> MSRQSISLRFPLLLLLLSPSPVFSADPGAPAPVNPCCYYPCQHQGICVRFGLDRYQCDCTRTGYSGPNCTIPEIWTWLRTTLRPSPSFIHFLLTHGRWLWDFVNATFIRDTLMRLVLTVRSNLIPSPPTYNIAHDYISWESFSNVSYYTRILPSVPRDCPTPMGTKGKKQLPDAEFLSRRFLLRRKFIPDPQGTNLMFAFFAQHFTHQFFKTSGKMGPGFTKALGHGVDLGHIYGDNLERQYQLRLFKDGKLKYQMLNGEVYPPSVEEAPVLMHYPRGIPPQSQMAVGQEVFGLLPGLMLYATIWLREHNRVCDLLKAEHPTWGDEQLFQTARLILIGETIKIVIEEYAQQLSGYFLQLKFDPELLFGAQFQYRNRIAMEFNQLYHFHPLMPDSFRVGPQDYSYEQFLFNTSMLVDYGVEALVDAFSRQPAGRIGGGRNIDHHILHVAVDVIKESRVLRLQPFNEYRKRFGMKPYTSFQELTGEKEMAAELEELYGDIDALE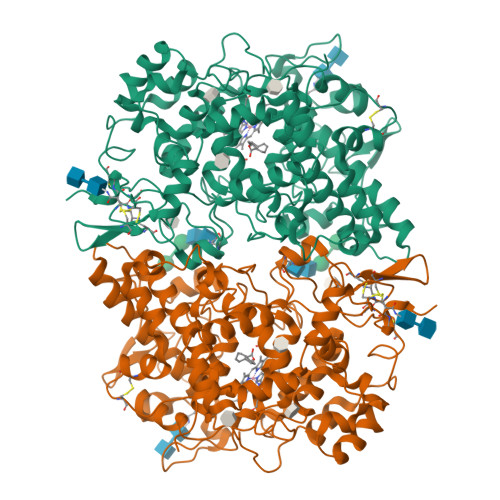FYPGLLLEKCHPNSIFGESMIEMGAPFSLKGLLGNPICSPEYWKASTFGGEVGFNLVKTATLKKLVCLNTKTCPYVSFHVPDPRQEDRPGVERPPTEL> SNASADAQSFLNRVCGVSAARLTPCGTGTSTDVVYRAFDIYNDKVAGFAKFLKTNCCRFQEKDEDDNLIDSYFVVKRHTFSNYQHEETIYNLLKDCPAVAKHDFFKFRIDGDMVPHISRQRLTKYTMADLVYALRHFDEGNCDTLKEILVTYNCCDDDYFNKKDWYDFVENPDILRVYANLGERVRQALLKTVQFCDAMRNAGIVGVLTLDNQDLNGNWYDFGDFIQTTPGSGVPVVDSYYSLLMPILTLTRALTAESHVDTDLTKPYIKWDLLKYDFTEERLKLFDRYFKYWDQTYHPNCVNCLDDRCILHCANFNVLFSTVFPPTSFGPLVRKIFVDGVPFVVSTGYHFRELGVVHNQDVNLHSSRLSFKELLVYAADPAMHAASGNLLLDKRTTCFSVAALTNNVAFQTVKPGNFNKDFYDFAVSKGFFKEGSSVELKHFFFAQDGNAAISDYDYYRYNLPTMCDIRQLLFVVEVVDKYFDCYDGGCINANQVIVNNLDKSAGFPFNKWGKARLYYDSMSYEDQDALFAYTKRNVIPTITQMNLKYAISAKNRARTVAGVSICSTMTNRQFHQKLLKSIAATRGATVVIGTSKFYGGWHNMLKTVYSDVENPHLMGWDYPKCDRAMPNMLRIMASLVLARKHTTCCSLSHRFYRLANECAQVLSEMVMCGGSLYVKPGGTSSGDATTAYANSVFNICQAVTANVNALLSTDGNKIADKYVRNLQHRLYECLYRNRDVDTDFVNEFYAYLRKHFSMMILSDDAVVCFNSTYASQGLVASIKNFKSVLYYQNNVFMSEAKCWTETDLTKGPHEFCSQHTMLVKQGDDYVYLPYPDPSRILGAGCFVDDIVKTDGTLMIERFVSLAIDAYPLTKHPNQEYADVFHLYLQYIRKLHDELTGHMLDMYSVMLTNDNTSRYWEPEFYEAMYTPHTVLQ;> SNAAIASEFSSLPSYAAFATAQEAYEQAVANGDSEVVLKKLKKSLNVAKSEFDRDAAMQRKLE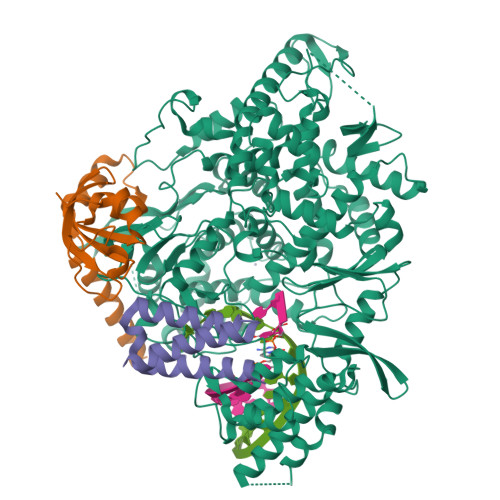KMADQAMTQMYKQARSEDKRAKVTSAMQTMLFTMLRKLDNDALNNIINNARDGCVPLNIIPLTTAAKLMVVIPDYNTYKNTCDGTTFTYASALWEIQQVVDADSKIVQLSEISMDNSPNLAWPLIVTALRANSAVKLQ;> SNASKMSDVKCTSVVLLSVLQQLRVESSSKLWAQCVQLHNDILLAKDTTEAFEKMVSLLSVLLSMQGAVDINKLCEEMLDNRATLQ>[8x]GSHMSASAELEPDVKGRILDAAADAFMARGFANTTIDDIADEVGATKGLIYYHFRSKFDIFLAVYEDGMRRVRERVEPHSTAPGTGHQRLEAMSIAHLENLMTELGYHHVVHQGVRHQDSTALKVRQRDALTALNELRRDYERMFRRVIAEGIADGSLRRVDEALATRTLLSNLNAVDVWYRKIEGQTGEEIRELASQVVDMLIGGLAD

The mycobacterial repressor, DarR, a TetR family regulator (TFR), was the first transcription regulator shown to bind c-di-AMP. Recently, DarR, a 201 residue, TFR regulator of a putative MDR transporter, Ms5347, in Mycobacteria was discovered and represents the focus of this work. Structures of TFR proteins reveal that they share a two-domain architecture with an N-terminal DNA-binding domain and a C-terminal inducer binding/dimerization domain. The DarR N-terminal domain consists of helices 1-3 and the dimer domain is comprised of helices α4-α9. In DarR, dimerization is mediated by helices α8 and α9, which interact with α8´ and α9´ (where the prime indicates the other subunit in the dimer) to form a four-helix bundle dimerization module.

However, to deduce the molecular mechanism of operator recognition by DarR, we next determined the structures of the Rhodococcus sp. USK13 and M. baixiangningiae DarR proteins in complex with a 20 bp site containing a double stranded (ds) DarR DNA operator, 5´-TAGATACTCCGGAGTATCTA-3´ (annealed to its complement). The structure of the Rhodococcus sp. USK13 DarR-DNA complex was solved first by selenomethionine SAD and refined to 2.96 Å resolution. This structure was then used to determine the 3.49 Å resolution structure of the M. baixiangningiae DarR-DNA complex. The Rhodococcus sp. USK13 DarR-DNA complex showed a pair of interacting DarR dimers in complex with the DNA (herein referred to as dimer-of-dimers) in the ASU while the M. baixiangningiae DarR-DNA structure contains two such complexes. These DarR-DNA complexes show the identical DNA binding mode, whereby the dimer-of-dimers partially encase the DNA using an electropositive surface. The same protein-DNA contacts are observed in the Rhodococcus sp. USK13 and M. baixiangningiae DarR-DNA structures. The distance between DarR recognition helices was found to be 39 Å for both DNA bound Rhodococcus sp. USK13 and M. baixiangningiae DarR dimers. By contrast, our DarR-DNA structures reveal that the centrally bound subunits of each of DarR dimer makes critical inter-subunit contacts. These β-sheet like interactions are formed between residues 116-125 of each subunit. Notably, these residues are adjacent to residues that interact with the inducer ligand in the M. baixiangningiae DarR structure and hence would be subject to allosterism.>MPRVKSYTGGTINFKEIESHLVGSSATARKDAVEALIAYFDGSRTQSQTTFDDKAYHRLFEALFRCTLIEKEAYFNSKKSVKVTAAAAARLERCPEALRLAVRHGVTTIRRKTARAIIDHIVQVLPGPDGAYVMPLLAGYVKVLYEFLDNPASAENIAALSGEGWEVCVDFCIDVLSRFLELGDRESGSLSRASPAPGATARSGSVAGTQGSGEQIGTHVAVDVLSCLYMLCIAHNAPIQRKADRLPHVVIQLLQLRQMKIGELQKMAFATFNIVFQRMQAEDVALCKTLVKQVVPLLSHWWQPRALSRDAMLNSIRDEMLKTLYGTRLYIQALLREAADESFPQDVEELLDTLWCDYSRREERARLQLDDITFTNMLLPPDHPRTGIFSLRPHHTAGEQNWALLENLAILEAAYSKHGQQEQSQQNQQQPEIDQPRKRRKMSGRQNRVHQKLHSLDPAVRLSALQLIPFLTRHKKPSLEDVAETLEDLSKHVTAKQAIVASWAMLACSSLAIHEVSRHPSLSSSWKQLWQLAVRSLSLPPISRASCVLLNSILKANLIPRHELADDINQIVTTADISGPAILVDASLGLMLNLLRFRNNMFPNASQATSNHIIRWVFVRWSPAELTYASLHGTHATPYDLVNLLRACYGISPLVMAQPLRLFNGPIVLHWKEQAEMEPFIRYLLLLHEEEPDTTVTPAQQEEQLPESNSATDVAGSNASRRLALELFYPKVEELQELAESWQKRGGEGATPVSMERLRSMVLACLTGALLLPDLVNINSSLSRDLESAVFSIVDATLKVILNSPPSENLFGMILASSAPYIPHLIEPELIALKRERPHLLKFFGKLSEALYERSRRESSHRDDQVIDIDPDFEPQTSQKNTASKAKTLPRRDILLSYTPEAFYLETSLRIHFLDIIRLNDGEIGRIPEPIINQLAGLSGEQFLCCREFMREIFTSDAIVPLGGATTILETAGHIVSRYEYACCEVALCNCIDIMDSFINLWTDNHFDIAEMAGDLYHYLVKQSLPNNSMSAAAQIRLASLLLHLLEVKSEYASNLGLPSSQSTLLKILQDGPMKLKHYIGLEIPKLFGLYVLKTHDDIFVDVLEHLPSDPDVVEGLAFRLFVLAELACRWPTLLRRSIYHTFEIPGKITKISKSQSCVTHSALYAASCIKRIAQTLKLSGPQELFKLFAPQLLYTWLDNDSIQDIAYEIFGFSSLLDLLREAQTEAAAIMMMRGQEQEVCQLAQSLGLTPEKLVQQSFTKIIAYSIAHDISIAGGPDYVTGESRMRKILGKEEYLANIHLNFADIISTFFDIFDQEDPIEKAFRRDERFAYAAETLEEIKKLGHLPTALPPNQQPMFRAKYLPREIVHLCSRTQYEPENIWTPALVVFVARKLLKTIHPALGPLHACSVLRKIRVLICLAGDHAISGYPLEMLLHSLRVFVVDPECADDALGITQYLIKRGDEYLKRTPSFLAGYALSSLADLRVFLESSQSSTTQESQFKATKSKAQEFHAWFSKYLAAYDSPEFKDEGQKQAFRS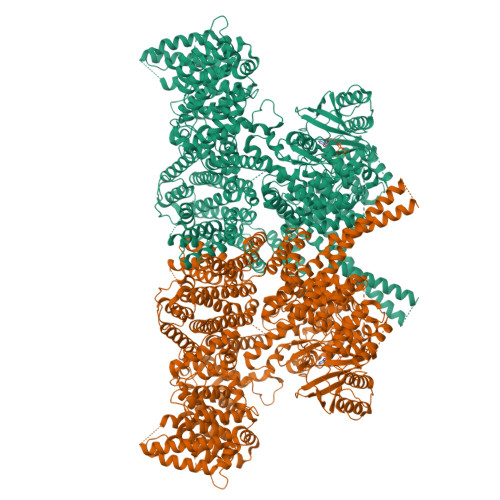ITENAAHIRASGNAEKGTHESNLLLEILKDWGRENQLLNEPARDVALSMLCGVFNIPPSSRLDVIETDEDAIKNGAVVWKSCSSQRLGGEYLAWAGRVLGRSFAASGEVPEDLLRESQLQEYRRLSQGVGSSEEGLLNLIKSLTISGDCFTAGLAEAALRTIVSDAISDNDHDLLSACQESLPEPLLIASNWDPYRTPLSDQFKVDPPANTEVFSARALENPNWSQHLAIRLALSAPKIVTLRVLPPILSKVKGFAERAFPFVVHLVLAYQLDKQQSAKRELSESLQEWLNFTSEPAKENLKLLINTILYLRTQPLPGESSIADRAHWLDVNMASAAAAATRCGMYKVALLFAELAAESTRGSRRSSAARETDDSSDILLEIFENIDDPDAYYGLSQDASLSTVLARLEYENDGAKSLAFRGAQYDSHLRGRDLQSRQDCNALIKALSSLGLAGLSNSLLQSQQSIDGSSDSLDATFTTARKLEIWNLPAPVNSDSWAVTVYKAYQSMYQAQELDTVRSMVHDGLKNTVRHLSSGSLNTSVLRQQLGALAALTELDDILNVRDQSELQCTLATFEKRSKWMMSGRYADVSQILSCRETTLSMWSQRHNLRAAGLTSADARLVQIRGMLLSSDIFRFHRARQETLNLSTALSDLIPSCESLGLSVDAAIKMEAANALWDHGEMISSIRMLQAIDKDSSLKKQSVPLSRSDLLSKIGYQVSVARLESPDAIQKKYLEPALKELKGKIEGREAGQVFHQFAVFCDEQLQNPDSLEDLARLQNLKKGKDEEVAQLKALIASAKDSQLRNRYQSHLAKAKQWQELDQQELRRVEQTRSEFLKLCIENYLLSLAASDEHDNDALRFMALWLEKSEEEVANEVVKKWINKVPTRKFALLMNQLSSRLQDHNTLFQKLLIDLVYRICVDHPYHGMYHIWTGARTRVNKDDEVAVSRQRATDKIAKALSKNNKVSSIWPAIDQTSRVYHALAMDRDPTRYKSGQKVPIKNSPVGQNFLSTMSNNPIPPPTLQIEVSANLDYSHVPMIHKFAPEMAIASGVSAPKILTAIGTDGRKYKQLVKGGNDDLRQDAIMEQVFAAVSELLKLHRETRQRNLGIRTYKVLPLTSSSGLIEFVSNTIPLHEYLMPAHERYYPKDLKGSQCRKEIANAQTKNTETRIAVYRRVTERFHPVMRYFFMEYFPDPDEWFQKRTNYTRTTAAISMLGHVLGLGDRHGHNILLDHKTGEVVHIDLGVAFEMGRVLPVPELVPFRLTRDIVDGMGITKTEGVFRRCCEFTLDALREEAASIQTILDSLRHDTLYQWSISPVRMAKLQNAREVGGEDGGVGGGEDGEGGGVPKEKKQRPANEPSEADRAIEVVKKKLSKTLSVMATVNDLINQATSVSNLAVLYSGWAAYA[2x]>[2x]HHHHHHMEPACKYDFATSVLFTEAELHTRMRGVAQRIADDYSNCNLKPLENPLVIVSVLK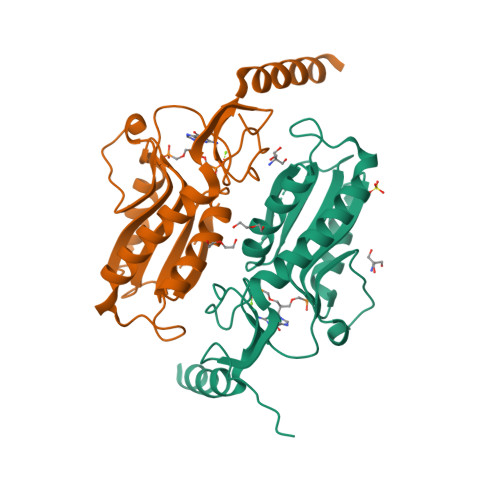GSFVFTADMVRILGDFGVPTRVEFLRASSYGHDTKSCGRVDVKADGLCDIRGKHVLVLEDILDTALTLREVVDSLKKSEPASIKTLVAIDKPGGRKIPFTAEYVVADVPNVFVVGYGLDYDQSYREVRDVVILKPSVYETWGKELERRKAAGEAKR> MLRDLFDRAVVLSAYIHNLSSEMF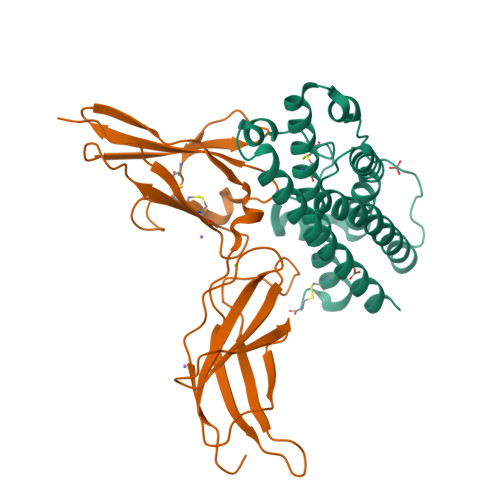SEFDKRYTHGRGFITKAINSCHTSSLATPEDKEQAQQMNQKDFLSLIVSILRSWNEPLYHLVTEVRGMQEAPEAILSKAVEIEEQTKRLLERMELIVSQVHPETKENEIYPVWSGLPSLQMADEESRLSAYYNLLHCLRRDSHKIDNYLKLLKCRIIHNNNC;> MLPPGKPEIFKCRSPNKETFTCWWRPGTDGGLPTNYSLTYHREGETLMHECPDYITGGPNSCHFGKQYTSMWRTYIMMVNATNQMGSSFSDELYVDVTYIVQPDPPLELAVEVKQPEDRKPYLWIKWSPPTLIDLKTGWFTLLYEIRLKPEKAAEWEIHFAGQQTEFKILSLHPGQKYLVQVRCKPDAGYWSAWSPATFIQIPSDFTMND> MADIGSEFYTLNWQPPYDWSWMLGFLAARAVSSVETVADSYYARSLAVGEYRGVVTAIPDIARHTLHINLSAGLEPVAAECLAKMSRLFDL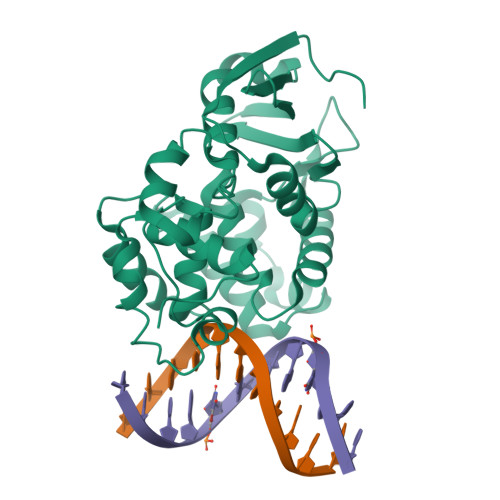QCNPQIVNGALGRLGAARPGLRLPGCVDAFEQGVRAILGQLVSVAMAAKLTARVAQLYGERLDDFPEYICFPTPQRLAAADPQALKALGMPLKRAEALIHLANAALEGTLPMTIPGDVEQAMKTLQTFPGIGRWTANYFALRGWQAKDVFLPDDCLIKQRFPGMTPAQIRRYAERWKPWRSYALLHIWYTEGWQPDEA>DEPNQPSTPEAVTKTVTIDASKYETWQYFSFSKGEVVNVTDYKNDLNWDMALHRYDVRLNCGESGKGKGGAVFSGKTEMDQATTVPTDGYTVDVLGRITVKYEMGPDGHQMEYEEQGFSEVITGKKNAQGFASGGWLEFSHGPAGPTYKLSKRVFFVRGADGNIAKVQFTDYQDAELKKGVITFTYTYPVK[2x]

In P. gingivalis, heme is primarily imported by heme-binding protein, HmuY, and its cognate outer-membrane receptor, HmuR. HmuY is an outer-membrane-associated lipoprotein, which is identical in sequence to a P. gingivalis envelope protein designated fibroblast activating factor. The protein is functional as a dimer in its heme-depleted form and as a tetramer once heme is bound. Structure similarity searches following a variety of algorithms failed to identify significant matches extending beyond selected parts of the central β-sandwich, so we conclude that HmuY conforms to a novel all β-fold.

In addition, we solved the X-ray crystal structure of holo-HmuY. The structure of HmuY is asymmetric, with maximal dimensions of ∼55×40×35 Å, and it resembles a right hand. It consists of a roughly globular nucleus reminiscent of a palm, out of which protruding segments mimicking thumb and fingers emerge. As anticipated by CD spectroscopy (see above and [23]), HmuY is an all β-protein constituted by 15 β-strands. A single Fe3+-chelating heme b molecule (hemin) is inserted laterally like a wedge into the cavity, curiously with its charged propionate substituents pointing toward the palm and the hydrophobic methyl and vinyl substituents pointing toward the exterior. However, the most relevant contacts are the metallo-organic bonds established between the heme iron and the Nε2 atoms of His134 (2.04 Å away), provided by thumb-strand β8, and His 166 (2.09 Å), from ring-finger-strand β11. These two ligands occupy the apical positions of an octahedral iron co-ordination sphere, whose equatorial ligands are the four porphyrin nitrogen atoms (at 2.03–2.06 Å). The quaternary structure of holo-HmuY is a cross-like tetramer of complexes, ∼95 Å in diameter, created by the combination of a local and a crystallographic two-fold axis. The overall arrangement entails that the four heme groups are in direct contact with each other in the center of the tetramer.> MDKTGWITHCFGRFLIDLPPDAVINAGYYLWGDRIEYLDDKPTELAARVDRLEQEWRTQRHKSKGNMFLRKIDFGNESVGLLSWSSEVASKTYLLDTYVTSKPTWHVYRWKGKVSVDREQHAVEISRALARNLRSRAPKEIPSEPGFCIDHAYIAGDSFQVERFGVGVTFPEHPGARFEFRSSTGAELNSLLERVDGFVQNMLSTFAGMETLRKGKHPVGSLPGEEYLVAGSDKGQRGYTFMWEV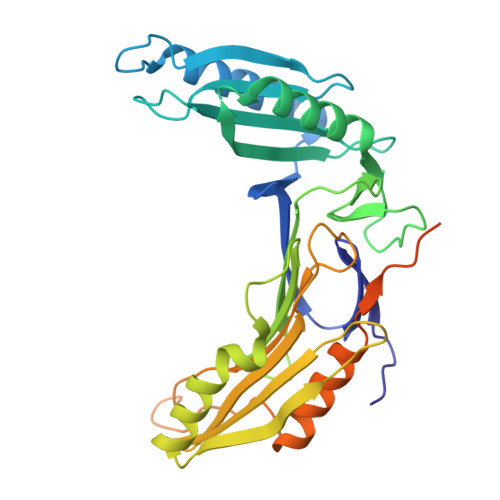QGKEESLTEPNLTAGLAVLERSNENGKPPPPAFKSDKEALELWDTIVDSIRVRPTSSSPRGGNAGPSPAPKPATPGGQTLGDHYVYEEFLSSLKPKDSWLDDL>QAEWRSWEVNKRLEYSLVKGITEFIEQDTEEARQQATRPIEVIEGPLMDGMNVVGDLFGEGKMFLPQVVKSARVMKQAVAYLEPFIEASKEQGKTNGKMVIATVKGDVHDIGKNIVGVVLQCNNYEIVDLGVMVPAEKILRTAKEVNADLIGLSGLITPSLDEMVNVAKEMERQGFTIPLL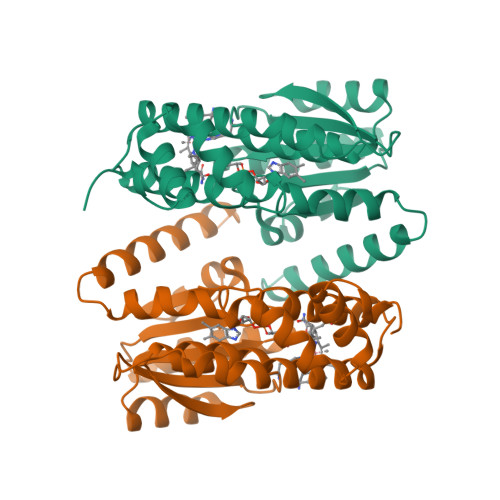IGGATTSKAHTAVKIEQNYSGPTVYVQNASRTVGVVAALLSDTQRDDFVARTRKEYETVRIQHGR[2x]>[4x]MKFTPPPSSLRGPLVIPDKIMMGPGPSNCSKRVLAALNNTCLSNFHDELFQVIDEVKDGLRYIFQTENRTTMCITGSAHTGMEALLCNLLEEGDIVLIANNGIWAERAINMATRYGADV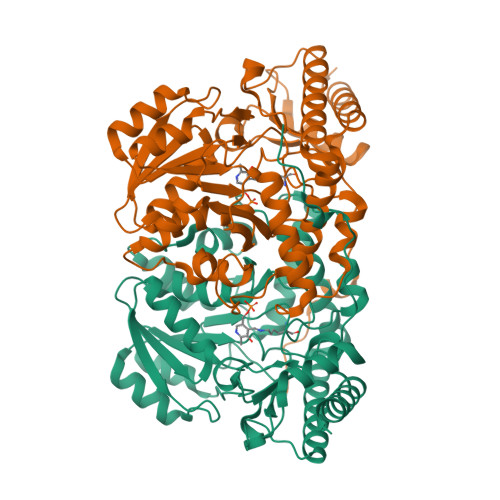RVLEGPADKPFSMTDFKKAIEQHRPKCLFVVHGDSSSGLLQPLEGLGKICHDYDCLLLVDAVASLCGVPFYMDKWEIDGVYTGSQKVLGAPPGITPISISPKALEVIRSRKTPSKVFYWDLLILGNYWGCYDEQKRYHHTVPSNLIFALREAIAQIAEEGLEPVIRRRQECAEQMYRGLQAMGLEIFVKDPEYRLPTVTCIMIPKGVNWWKVSEYAMNNFSLEIQGGFGPTMGIAWRAGIMGESSTLQRVNFYLYAFKESLKATHPD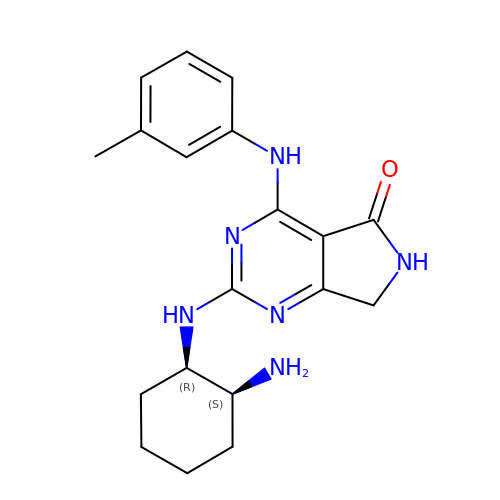2-{[(1R,2S)-2-aminocyclohexyl]amino}-4-[(3-methylphenyl)amino]-6,7-dihydro-5H-pyrrolo[3,4-d]pyrimidin-5-one | C19 H24 N6 O | VPNLOOYVNORYBV-UONOGXRCSA-N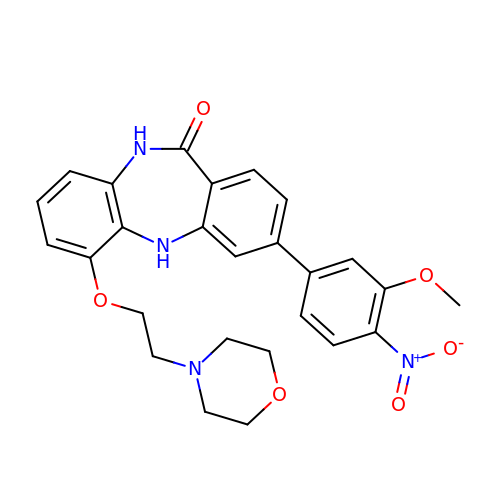3-(3-methoxy-4-nitrophenyl)-6-[2-(morpholin-4-yl)ethoxy]-5,10-dihydro-11H-dibenzo[b,e][1,4]diazepin-11-one | C26 H26 N4 O6 | FNAOLRABVJJTRC-UHFFFAOYSA-N> ADKELKFLVVDDFSTMRRIVRNLLKELGFNNVEEAEDGVDALNKLQAGGYGFVISCWNMPNMDGLELLKTIRADGAMSALPVLMVIAEAKKENIIAAAQAGASGYVVK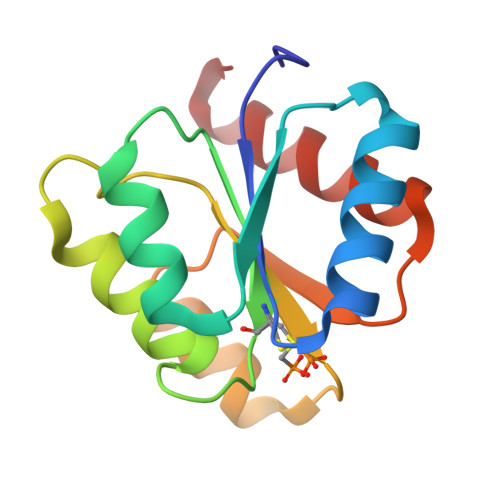PFTAATLEEKLNKIFEKLGM> 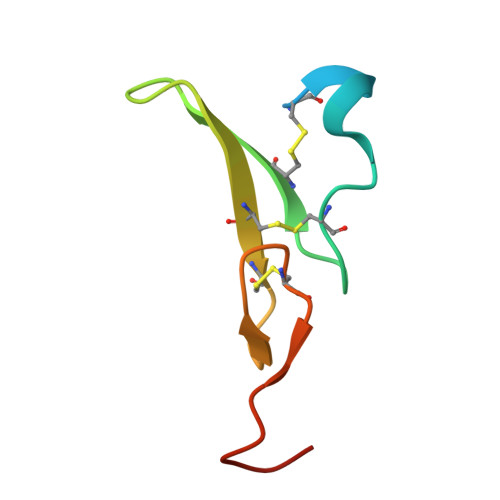GPTANSDSECPLSHDGYCLHDGVCMYIEALDKYACNCVVGYIGERCQYRDLKWWELR> MRRCSFASTCRYRSADDVPLGLGSAYVWTCRNITSRGQFNPIHNFSYAMERGVRARDVKAFEKLITNPGPLRVAYTPDYLDWLHRCYKAKGTYMDARAVAEKKFNGNIVSSELSAAVNRREGKRGDTRGDTVDNDHHNLPGAPPPGMFLRPAHSFRRLAGELKRRRAQSILDEVARAQGMLDLFERQPHFPAIHIDRCSRFHLVELFKEMVLERSLDSNMIWEKALLYRAILSERKPSYPTSFHYIFTAVEDTVFAPTISTPMEMAGSGGEGHDRSSHPLAAKCPTLEAYYYYVYLVKKYYIDNAVE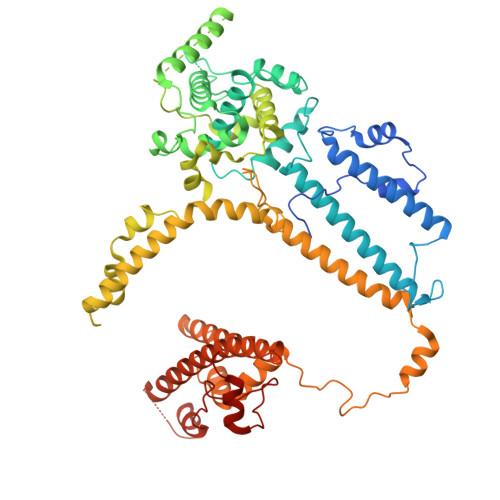AHVVLRCHREPNAADLLFSNPPPKDDTEIMKAVELLRNADIQRGVAAAAAVSDPTLPPGGEGSVIGNSDNXKNSEKXSEGSRGRPARPPVLPGAYPPIDMLWRCEENLPLLKVLLFGEFNLIVSENPFVKFPSAHGFLTRPYSTDSSRTLADGMSLANVMAEKRGHLLPSLPRNTATSIDARAQDIRRLQQKHHRDDIVSFQKLLRSTHAEDSPSAFSSYSDWSYFNPRAVRAEERDRLTRKAVEALKLYDSATNDIYRHSFEDVQACHTQRVTERDRTMPPYLPTLPHFVAIIKKDPHISFLLHIGLPDRNSSEEGSAKHKELEKRIYYLARALYHTALEYHNETVRRVNRQKVNVAASLLDNFVEQEWTTILRDKHDVTDVTKTLNDTQNDKKQLARRLGRYMLFANRSLDDTGFPTDARADDYTRWMAPPSVGKVSL> MGSSELNRKLVGYFPEWAYSSEAQGYFNVTDLQWDSLTHIQYSFAMVDPSTNKITLSNKHAAIEEDFSEFDLNYNGKKIELDPSLPYKGHFNVLQTMKKNYPDVSLLISVGGWTGTRCFYTMIDTDNRINTFADSCVDFIRKYGFDGVDIDFQYPSSTSQSGNPDDFDLSEPRRTKLNERYNILIKTLREKIDMASKEDGKEYLLTAAVTASPWVLGGISDNTYAKYLDFLSIMSYDYHGGWNEYVEHLAGIYPNKEDRETVTQIMPTLCMDWAYRYYRGVLPAEKILMGIPYYTRGWENVQGGINGLHGSSKTPASGKYNILGDDLNNDGVLEPAGANPLWHVLNLMEQDPNLKVYWDEISKVPYVWQNDKKVFVSFENEKSIDARLEYIQNKNLGGALIWVMNGDYGLNPNYVEGSNKINEGKYTFGDTLTKRLSQGLKKMGVCNKTPDDLNISLEPINVDVKFNGKYDHPNYTYSIDITNYTDKEIKGGWNVSFDLPKSAVFKSSWGGTYSVTDNGDFNTITLTSGAWQNIAPNSTITVQGMIGLCFSGIRNVTFNGMNPIGNDKSHHHHHH

C. perfringens type G, the causative agent of necrotic enteritis in broilers, produces two glycosyl hydrolase family 18 chitinases, ChiA and ChiB, which display distinct substrate preferences. Whereas ChiB preferentially processes linear substrates such as chitin, ChiA prefers larger and more branched substrates, such as carbohydrates presented by the chicken intestinal mucus. Here, we show via crystal structures of ChiA and ChiB in the apo and ligand-bound forms that the two enzymes display structural features that explain their substrate preferences providing a structural blueprint for further interrogation of their function and inhibition. We succeeded in obtaining several crystal structures of recombinant ChiA and ChiB in apo (unbound) and ligand-bound forms to resolutions between 1.30 Å and 1.85 Å. Both ChiA and ChiB encode for an N-terminal glycosyl hydrolase family 18 (GH18) Trios-phosphate Isomerase (TIM) barrel followed by a C-terminal putative carbohydrate binding domain (CBD).

The E196Q point mutant of ChiA was generated to capture the ligand within a co-crystal structure. E196 is expected to be protonated in the catalytically competent state and act as a general acid/base to protonate the glycosidic bond during the substrate hydrolysis. In the first, bound conformation, the oligosaccharide has descended towards the active site occupying positions -2 to +3. The GlcNAc at position -1 is in the boat conformation, priming it for the formation of the oxazolinium reaction intermediate. In the second, encounter conformation, the elongated oligosaccharide is located at the surface of the cleft and only engages the CBM side of the cleft. Overall ChiA displays the hallmarks of a chitinase processing chitin from its non-reducing end towards the reducing end.>VNTTLFRWPVRVYYEDTAAGGVVYHASYVAFYERARTEMLRHHH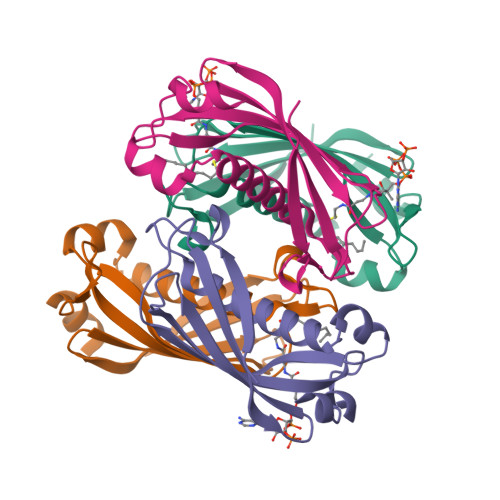FSQQALMAERVAFVVRKMTVEYYAPARLDDMLEIQTEITSMRGTSLVFTQRIVNAENTLLNEAEVLVVCVDPLKMKPRALPKSIVAEFKQ[4x]> MGQNTLKVHDLNEDAEFDENGVEVFDEKALVEEEPSDNDLAEEELLSQGATQRVLDATQLYLGEIGYSPLLTAEEEVYFARRALRGDVASRRRMIESNLRLVVKIARRYGNRGLALLDLIEEGNLGLIRAVEKFDPERGFRFSTYATWWIRQTIERAIMNQTRTIRLPIHIVKELNVYLRTARELSHKLDHEPSAEEIAEQLDKPVDDVSRMLRLNERITSVDTPLGGDSEKALLDILADEKENGPEDTTQDDDMKQSIVKWLFELNAKQREVLARRFGLLGYEAATLEDVGREIGLTRERVRQIQVEGLRRLREIL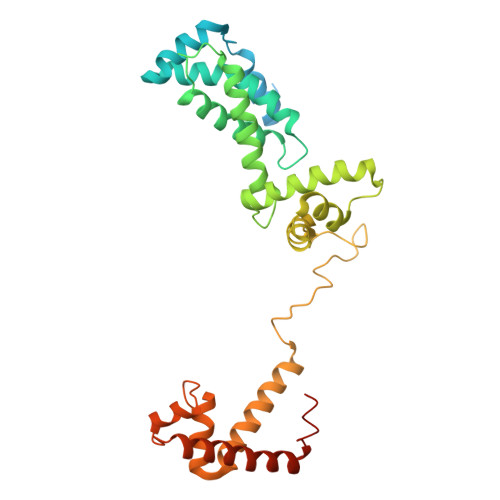QTQGLNIEALFLEHHHHHH>GSTMSLSRSEEMHRLTENVYKTIMEQFNPSLRNFIAMGKNYEKALAGVTYAAKGYFDALVKMGELASESQGSKELGDVLFQMAEVHRQIQNQLEEMLKSFHNELLTQLEQKVELDSRYLSAALKKYQTEQRSKGDALDKCQAELKKLRKKSQGSKNPQKYSDKELQYIDAISNKQGELENYVSDGYKTALTEERRRFCFLVEKQCAVAKNSAAYHSKGKELLAQKLPLWQQGVDSSG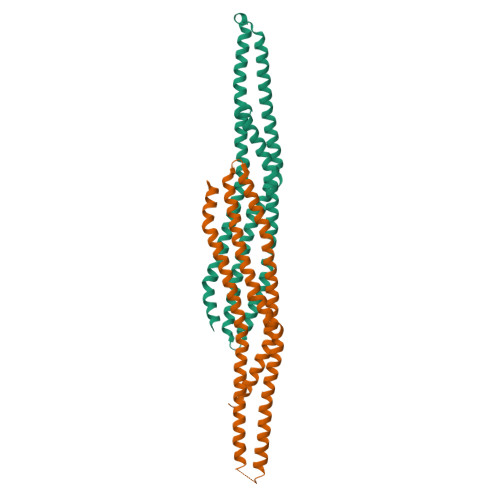RIVTD[2x]>[2x]MSLYDVTEWKHVFKLDPNKDLPDEQL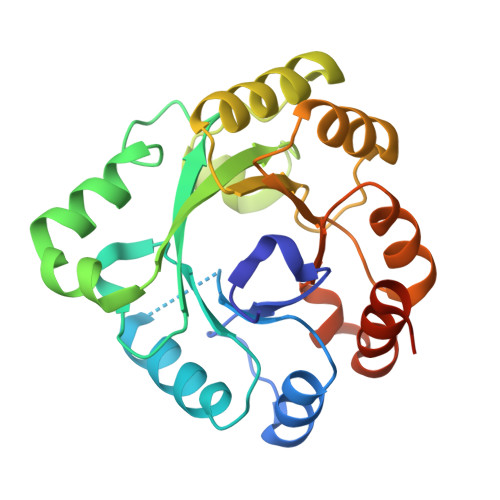EILCESGTDAVIIGGSDGVTEDNVLRMMSKVRRFLVPCVLEVSAIEAIVPGFDLYFIPSVLNSKNADWIVGMHQKAMKEYGELMSMEEIVAEGYCIANPDCKAAALTEADADLNMDDIVAYARVSELLQLPIFYLEYSGVLGDIEAVKKTKAVLETSTLFYGGGIKDAETAKQYAEHADVIVVGNAVYEDFDRALKTVAAVKGEEGGSHHHHHH> MGNVIDLGEYGARFTEDPYPVYAELRERGPVHWVRTPPPEAFEGWLVVGHEEARAALADPRLSKDGTKKGLTSLDVELMGPYLLVVDPPEHTRLRSLVARAFTMRRVEALRPRIQEITDGLLDEMLPRGRADLVD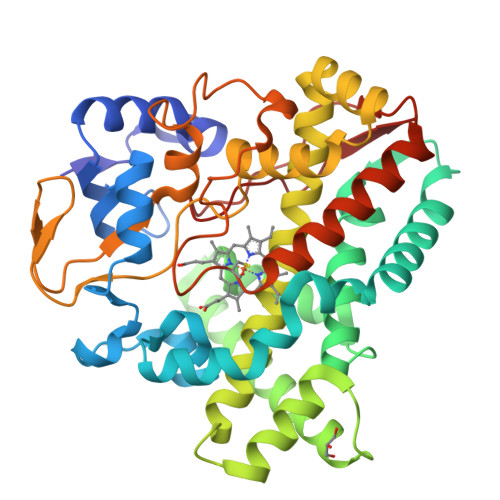SFAYPLPITVICELLGVPDIDRVTFRALSNEIVAPTGGDAELAAYERLAAYLDELIDDKRSTAPADDLLGDLIRTRAEDDDRLSGEELRAMAFILLVAGHETTVNLITNGVHTLLTHPDQLAALRADMTLLDGAVEEVLRFEGPVETATYRYAAESMEIGGTAIAEGDPVMIGLDAAGRDPARHPDPHVFDIHRAPQGHLAFGHGIHYCLGAPLARLEARVALRSLLERCPDLALDGPPGARPPGMLIRGVRRLPVRW>[4x]GDKDLGHIVKTIRCLEEEGHIDKSFRERFLTWYSLRATHR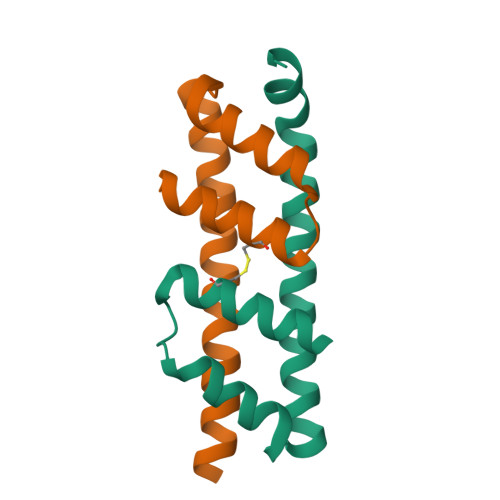EVRVVKDFVETFMEDLSSLGQQLVDTFSESILSKR> MGSSHHHHHHSQGSMERKISRIHLVSEPSITHFLQVSWEKT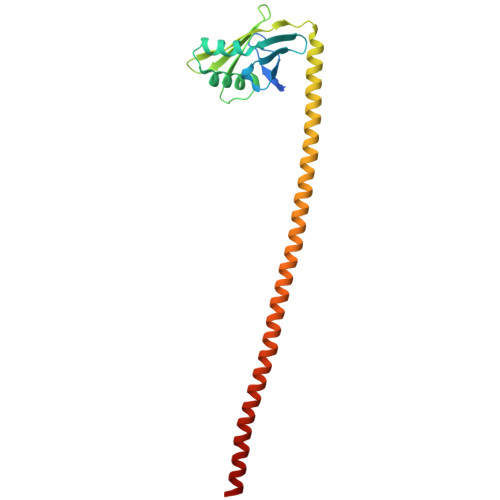LESGFVITLTDGHSAWTGTVSESEISQEADDMAMEKGKYVGELRKALLSGAGPADVYTFNFSKESCYFFFEKNLKDVSFRLGSFNLEKVENPAEVIRELICYCLDTIAENQAKNEHLQKENERLLRDWNDVQGRFEKCVSAKEALETDLYKRFILVLNEKKTKIRSLHNKLLNAAQEREKDIKQEG>GAMATVQDML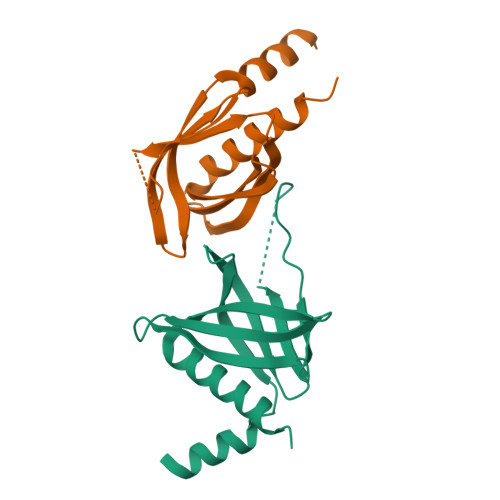SSHHYKSFKVSMIHRLRFTTDVQLGISGDKVEIDPVTNQKASTKFWIKQKPISIDSDLLCACDLAEEKSPSHAIFKLTYLSNHDYKHLYFESDAATVNEIVLKVNYILESRASTA[2x]> MIQGVIQKIAGPAVIAKGMLGARMYDICKVGEEGLVGEIIRLDGDTAFVQVYEDTSGLKVGEPVVSTGLPLAVELGPGMLNGIYDGIQRPLERIREKTGIYITRGVVVHALDREKKWAWTPMVKPGDEVRGGMVLGTVPEFGFTHKILVPPDVRGRVKEVKPAGEYTVEEPVVVLEDGTELKMYHTWPVRRARPVQRKLDPNTPFLTGMRILDVLFPVAMGGTAAIPGPFGSGKTVTQQSLAKWSNADVVVYVGCGERGNEMTDVLVEFPELTDPKTGGPLMHRTVLIANTSNMPVAAREASIYVGVTIAEYFRDQGFSVALMADSTSRWAEALREISSRLEEMPAEEGYPPYLAARLAAFYERAGKVITLGGEEGAVTIVGAVSPPGGDMSEPVTQSTLRIVGAFWRLDASLAFRRHFPAINWNGSYSLFTSALDPWYRENVAEDYPELRDAISELLQREAGLQEIVQLVGPDALQDAERLVIEVGRIIREDFLQQNAYHEVDAYCSMKKA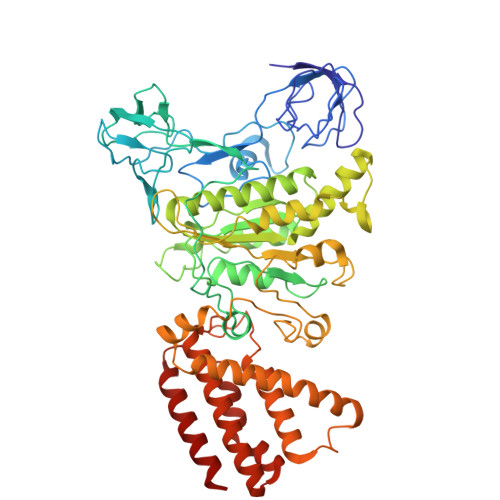YGIMKMILAFYKEAEAAIKRGVSIDEILQLPVLERIGRARYVSEEEFPAYFEEAMKEIQGAFKALA>[2x]MASSNLIKQLQERGLVAQVTDEEALAERLAQGPIALYCGFDPTADSLHLG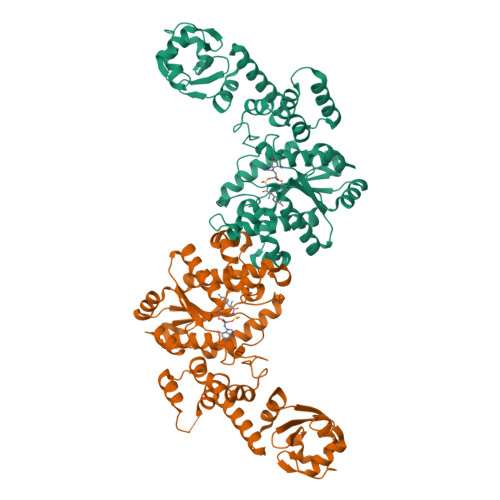HLVPLLCLKRFQQAGHKPVALVGGATGLIGDPSFKAAERKLNTEETVQEWVDKIRKQVAPFLDFDCGENSAIAANNYDWFGNMNVLTFLRDIGKHFSVNQMINKEAVKQRLNREDQGISFTEFSYNLLQGYDFACLNKQYGVVLQIGGSDQWGNITSGIDLTRRLHQNQVFGLTVPLITKADGTKFGKTEGGAVWLDPKKTSPYKFYQFWINTADADVYRFLKFFTFMSIEEINALEEEDKNSGKAPRAQYVLAEQVTRLVHGEEGLQAAKRITECLFSGSLSALSEADFEQLAQDGVPMVEMEKGADLMQALVDSELQPSRGQARKTIASNAITINGEKQSDPEYFFKEEERLFGRFTLLRRGKKNYCLICWK>[2x]MEFTTGLMSLDTALNEMLSRVTPLTAQETLPLVQCFGRILASDVVSPLDVPGFDNSAMDGYAVRLADIASGQPLPVA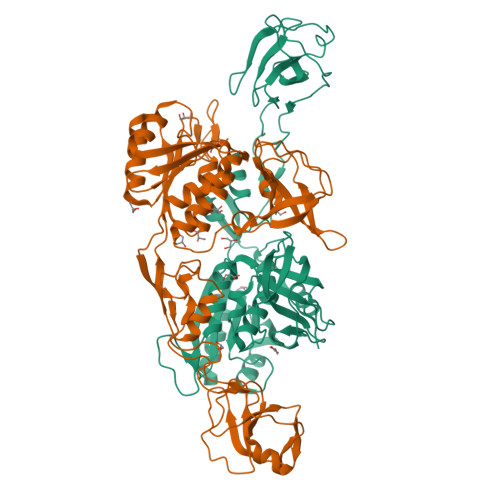GKSFAGQPYHGEWPAGTCIRIMTGAPVPEGCEAVVMQEQTEQMDNGVRFTAEVRSGQNIRRRGEDISAGAVVFPAGTRLTTAELPVIASLGIAEVPVIRKVRVALFSTGDELQLPGQPLGDGQIYDTNRLAVHLMLEQLGCEVINLGIIRDDPHALRAAFIEADSQADVVISSGGVSVGEADYTKTILEELGEIAFWKLAIKPGKPFAFGKLSNSWFCGLPGNPVSATLTFYQLVQPLLAKLSGNTASGLPARQRVRTASRLKKTPGRLDFQRGVLQRNADGELEVTTTGHQGSHIFSSFSLGNCFIVLERDRGNVEVGEWVEVEPFNALFGGL>QTRSSRMAGFGHAVPARCVDNAEIEASLGLEAGWIERRTGIRSRYWAEAGDTLSGLAERAG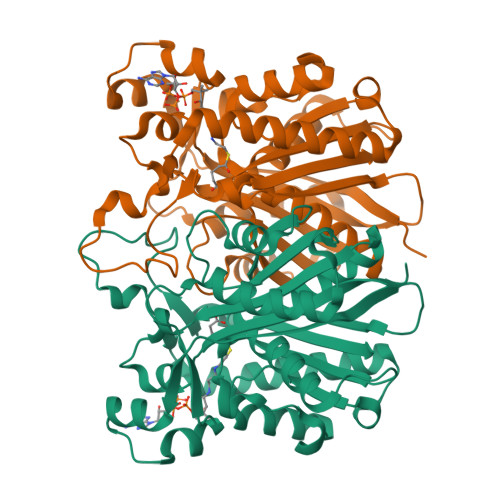RMALEDAKINADDIALTLLATSTPDHLLPPSAPLLAHRLGLTRSGAIDLAGASSGFLYALTLADGFVRTYGRAVLVVAANILSRRINPAERASAVLFADAAGAVVLTPCPEVKRGVLSADLVADGSGYDLIQIAAGGSSQPFSAGMIAEDALMTMRDGREVFSRAVALMTNTSQRVLHEAELTAADISRFVPHQANARMSDAVCGNLGIEREKTVRTIGSFGNSSAATIPLSLSITNAERPLAGGETLLLTAAGAGMTGGAVVYRV[4x]>[3x]MIRSMTAYARREIKGEWGSATWEMRSVNQRYLETYFRLPEQFRSLEPVVRERIRSRLTRGKVECTLRYEPDVSAQGELILNEKLAKQLVTAANWVKMQSDEGEIN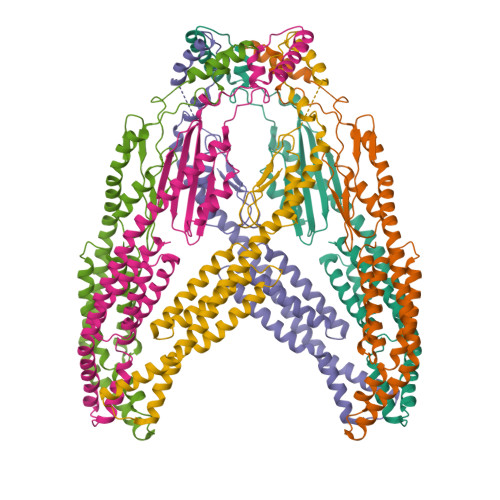PVDILRWPGVMAAQEQDLDAIAAEILAALDGTLDDFIVARETEGQALKALIEQRLEGVTAEVVKVRSHMPEILQWQRERLVAKLEDAQVQLENNRLEQELVLLAQRIDVAEELDRLEAHVKETYNILKKKEAVGRRLDFMMQEFNRESNTLASKSINAEVTNSAIELKVLIEQMREQIQNIE>GSYGSSSQSSSYGQPQSGSYSQQPSYGGQQQSYGQQQSYNPPQGYGQQNQYNSSSGGGGGGGGGGNYGQDQSSMSSGGGSGGGYGNQDQSGGGGSGGYGQGDRG[8x]

FUS (FUsed in Sarcoma) is a 54 kDa RNA-binding protein with multiple functions, including roles in the regulation of transcription through interactions with the C-terminal domain of RNA polymerase II8,9, in RNA splicing through multimeric binding to long introns, in DNA damage repair, in cellular responses to stress, and in mRNA transport and subcellular localization of translation. The N-terminal half is an LC domain comprised primarily of Ser, Gly, Gln, Tyr, Thr, and Pro residues, and with no Leu, Ile, Val, or Phe residues. Although the LC domain of FUS is largely unstructured as a monomer in solution, the LC domain is essential for normal FUS functions, including shuttling between the nucleus and cytoplasm, DNA damage repair, and transcription regulation. Phase-separated high-concentration droplets of full-length FUS or its LC domain typically evolve over time to a hydrogel state, consisting of highly entangled, amyloid-like fibrils, or to precipitated fibril bundles.

Here we report studies of the C-terminal half of FUS-LC (FUS-LC-C, residues 111–214). Although this segment is dynamically disordered in fibrils formed by full-length FUS-LC, we find that FUS-LC-C by itself readily forms highly ordered fibrils, suitable for molecular structure determination by cryogenic electron microscopy (cryo-EM). Three-dimensional (3D) helical reconstruction followed by 3D refinement with pseudo-21 symmetry yielded a final density map with 2.62 Å average resolution, based on the standard Fourier shell correlation criterion. The molecular model shows that residues 113–122, 135–136, and 139–149 form the β-strands of in-register parallel β-sheets. Residues 123–134 adopt an irregular conformation that allows the protein chain to fold back on itself. Side chains of most Gln residues in residues 112–150 are buried within the FUS-LC-C fibril core, with the sole exception of Q124. Thus, burial of Gln side chains appears to be a factor that determines the core structure. The interface between subunits also includes contacts between aromatic side chains of Y136 and Y143, possibly creating favorable π-stacking interactions. The absence of charged amino acid side chains and the absence of purely hydrophobic residues other than Pro within the FUS-LC-C fibril core implies that hydrophobic interactions and salt bridges do not account for the formation of FUS-LC-C fibrils.>MATLTAKNLAKAYKGRRVVEDVSLTVNSGEIVGLLGPNGAGKTTTFYMVVGIVPRDAGNIIIDDDDISLLPLHARARRGIGYLPQEASIFRRLSVYDNLMAVLQIRDDLSAEQREDRANELMEEFHIEHLRDSMGQSLSGGERRRVEIARALAANPKFILLDEPFAGVDPISVIDIKRIIEHLRDSGLGVLITDHNVRETLAVCERAYIVSQGHLIAHGTPTEILQDEHVKRVYLGEDFRL[2x];> MIIIRYLVRETLKSQLAILFILLLIFFCQKLVRILGAAVDGDIPANLVLSLLGLGVPEMAQLILPLSLFLGLLMTLGKLYTESEITVMHACGLSKAVLVKAAMILAVFTAIVAAVNVMWAGPWSSRHQDEVLAEAKANPGMAALAQGQFQQATNGSSVLFIESVDGSDFKDVFLAQIRPKGNARPSVVVADSGHLTQLRDGSQVVTLNQGTRFEGTALLRDFRITDFQDYQAIIGHQAVALDPNDTDQMDMRTLWNTDTDRARAELNWRITLVVTVFMMALMVVPLSVVNPRQGRVLSMLPAMLLYLLFFLIQTSLKSNGGKGKLDPTLWMWTVNLIYLALAIVLNLWDTVPVRRLRASFSRKGAV;> MQPFGVLDRYIGKTIFTTIMMTLFMLVSLSGIIKFVDQLKKAGQGSYDALGAGMYTLLSVPKDVQIFFPMAALLGALLGLGMLAQRSELVVMQASGFTRMQVALSVMKTAIPLVLLTMAIGEWVAPQGEQMARNYRAQAMYGGSLLSTQQGLWAKDGNNFVYIERVKGDEVLGGISIYAFNENRRLQSVRYAATAKFDPEHKVWRLSQVDESDLTNPKQITGSQTVSGTWKTDLTPDKLGVVALDPDALSISGLHNYVKYLKSSGQDAGRYQLNMWSKIFQPLSVAVMMLMALSFIFGPLRSVPMGVRVVTGISFGFVFYVLDQIFGPLTLVYGIPPIIGALLPSASFFLISLWLLMRKS

The IM component LptB2FG comprises an ATP-binding cassette (ABC) transporter, which powers the transport of LPS across the bridge. The cytoplasmic LptB dimer binds and hydrolyses ATP and the transmembrane (TM) domains of LptF and LptG create a cavity to accommodate LPS. LptB2 constitutes the cytoplasmic NBD dimer and the six TM helices of LptF and LptG (F_TM1-TM6 and G_TM1-TM6) constitute two TMDs that are arranged to form a central cavity with two surface gaps between TM1F and TM5G and TM1G and TM5F termed as lateral gates. To understand the mechanisms of how LptB2FGC recognises and acts to transport LPS, we obtained high-resolution cryo-electron microscopy (cryo-EM) structures of LptB2FGC complexed with substrate LPS or ATP analogue β-γ-imidoadenosine 5′-triphosphate (AMP-PNP).

We also obtained cryo-EM structure of LptB2FG complexed with LPS to compare the conformational changes with and without the presence of LptC. In this study, we used cryo-EM to resolve an LPS-bound structure of sfLptB2FG at overall 3.7 Å resolution with TM domain at 3.2 Å resolution. The cryo-EM maps of sfLptB2FG show clear side chain densities in the nucleotide-binding domains (NBDs) and the two transmembrane domains (TMDs), allowing us to unambiguously fit models of NBDs and TMDs of LptB2FG. The densities for the periplasmic domains of LptF and LptG are at low resolution but are clearly visible. The cryo-EM structure reveals a clear LPS density in the central cavity, showing all six acyl tails, glucosamine disaccharide phosphorylated at 1′ and 4′ positions, and the inner core oligosaccharide. The LPS molecule trapped is a natural substrate of sfLptB2FG that was overexpressed in the E. coli C43(DE3) strain. The acyl tails of LPS are drooped and perpendicular to the IM plane in the upper cavity and the inner core positioned above in the periplasmic space. In the cavity, hydrophobic residues I25, F26, L62, L66, L70 and M303 of LptF and L26, I33, I66, F67, I313, F317 and Y320 of LptG interact with the LPS acyl tails via van der Waals interactions. Charged residues K34, K62, R133 and R136 of LptG and R33 of LptF form salt bonds with the 1′-phosphate group of LPS, while K40 of LptG and K317 of LptF form salt bonds with the 4′-phosphate group of LPS. D37 of LptG interacts with the glucosamine disaccharide of lipid A. K322, R263 and Q248 of LptF and K41 of LptG interact with the inner core oligosaccharide.N-methyl-8-(1-methyl-2,2-dioxo-2,3-dihydro-1H-2lambda~6~,1-benzothiazol-5-yl)-1,6-naphthyridine-2-carboxamide 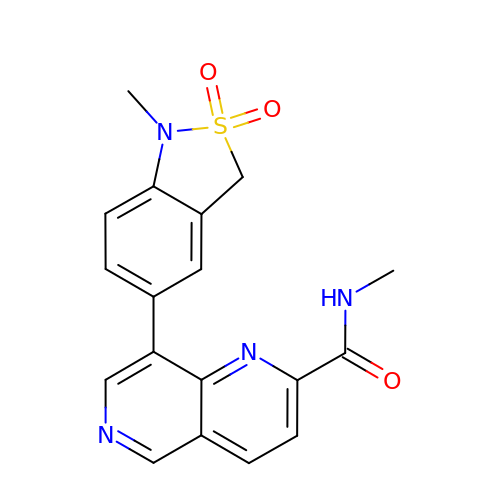| C18 H16 N4 O3 S | DFYVDBLGPYTIAT-UHFFFAOYSA-N> MANVNKVVRRRQVALLIALVLGIGAGGAGTWMVSEMNLKKAPPAKAPKGEPAPDMTGVVNQSFDNKVQRSAIAEAQRLNKETQTEIKKLRTEMGLVSRDLKGSQDRIRELEDQNQLLQTQLEAGKNFDSLSAEPLPGALASQGKPAPAGNVPPPTSFWPAGGGQAPAAPVMTPIQRPGMMDSQEFSLPDTGPKKPRFPWISSGSFVEAIVVEGADANASVTGDKNTAPMQLRLTGKVQMPNDEEFDLTGCFVTLEAWGDVSSERAIVRSRSISCKLGDDDIDQKIAGHVSFMGKNGIKGEVVMRNGQILLYAGGAGFLDGIGKGIEKASSTTVGVGATASMSAADIGQAGLGGGVSSAAKTLSDYYIKRAEQYHPVIPIGAGNEVTLVFQDGFQLETLEEARAKAAARKKQNQPSAS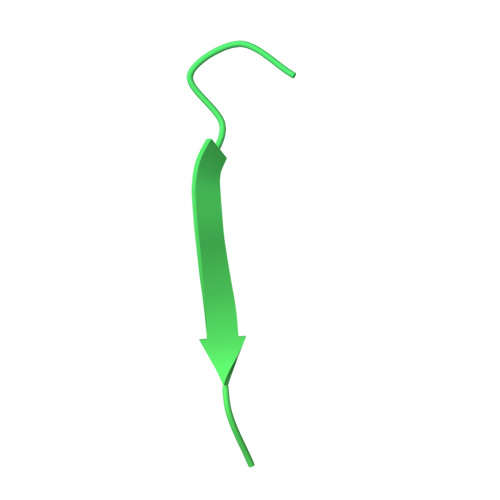STPAAMPGNTPDMLKQLQDFRVGDTVDPATGQVVTQ>MSDGTDQSDSGNAVQSAARVERAADGPGGSGGGGSGGGGVGVSTGSYDNQTHYKFLGDGWVEITAYSTRMVHLNMPKSENYCRVRVHNTNDTGTASHMAMDDAHEQIWTPWSLVDANAWGVWFQPSDWQYISNNMIHINLHSLDQELFNVVIKTVTEQNTGAEAIKVYNNDLTAAMMVALDSNNILPYTPAIDNQETLGFYPWKPTIPSPYRYYFSCDRNLSVTYKDEAGTITDTMGLASGLNSQFFTIENTQRINLLRTGDEYATGTYYFDTEPIRLTHTWQTNRHLGQPPQITELPSSDTANATLTARGYRSGLTQIQGRNDVTEATRVRPAQVGFCQPHDNFETSRAGPFKVPVVPADITQGLDHDANGSLRYTYDKQHGQSWASQNNKDRYTWDAVNYDSGRWTNNCFIQSVPFTSEPNANQILTNRDNLAGKTDIHFTNAFNSYGPLTAFPHPAPIYPQGQIWDKELDLEHKPRLHTQAPFVCKNNAPGQLLVRLAPNLTDQYDPNSSNLSRIVTYGTFFWKGKLTLKAKMRPNATWNPVFQISATNQGTNDYMSIERWLPTATGNITNVPLLSRPVARNTY[60x]

Members of the rodent protoparvovirus I species, including LuIII, H-1 parvovirus (H-1PV), and minute virus of mice (MVM), are utilized as replication-competent vectors to target cancer. The T = 1 icosahedral parvovirus capsids consist of 60 VPs, with the protoparvoviruses assembled from VP1 and VP2 in a 1:10 ratio. VP2 forms virus-like-particles (VLPs) for members of the protoparvoviruses that are otherwise antigenically and structurally equivalent to VP1/2/3 genome packaging capsids. LuIII kills transformed cell types that are either completely resistant, or less easily infected and lysed by H-1PV and MVM.

To enable comparative analysis for identifying the VP2 determinant of selective tumor tropism by the protoparvoviruses, the structure of LuIII VP2 VLPs was determined by cryo-electron microscopy and 3D image reconstruction (cryo-reconstruction) to 3.17 Å resolution. At this resolution, the VP2 amino acid side-chain conformations were unambiguously assigned into the cryo-reconstructed density map, from N-terminal residue 37 to the last C-terminal residue 587 (VP2 numbering). The LuIII VP2 monomer structure contains the core secondary structure elements reported for other Parvoviridae structures, with nine β-strands (βA-βI) and an α-helix (α-A). The conserved jellyroll motif contains eight antiparallel β-strands that form two β-sheets (β-BIDG and β-CHEF). The LuIII capsid is ~280 Å in diameter from 3-fold to 3-fold, similar to previous reports for H-1PV and MVM. In LuIII, this depression is 4–7 Å deeper, and 15–22 Å wider than H-1PV and MVM, respectively, resulting from multiple subtle side-chain differences within residues in VR5, VR6, and VR8. At the 3-fold axis, the single “windmill” shaped protrusion is the same height in all three viruses, but is narrower in LuIII compared to H-1PV and MVM, and has the same curvature for LuIII and H-1PV. At the 5-fold region, the depression appears wider in LuIII, due to a difference in the HI loop (VR7) residues that line the floor of the depression, and differential positioning of the apex of the DE loop (VR1) results in a 5-fold channel that is more open at the apex for LuIII.>[6x]MSLIDPRAIIDPSARLAADVQVGPWSIVGAEVEIGEGTVIGPHVVL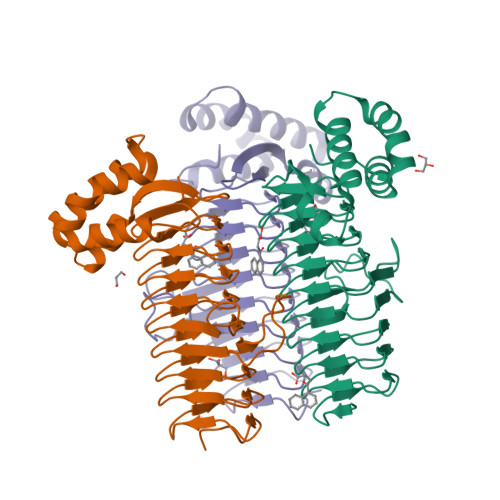KGPTKIGKHNRIYQFSSVGEDTPDLKYKGEPTRLVIGDHNVIREGVTIHRGTVQDRAETTIGDHNLIMAYAHIGHDSVIGNHCILVNNTALAGHVHVDDWAILSGYTLVHQYCRIGAHSFSGMGSAIGKDVPAYVTVFGNPAEARSMNFEGMRRRGFSSEAIHALRRAYKVVYRQGHTVEEALAELAESAAQFPEVAVFRDSIQSATRGITR> XIKQ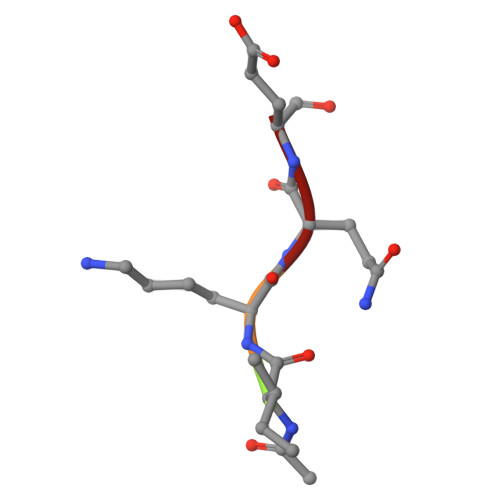E> GSMDEQEALNSIMNDLVALQMNRRHRMPGY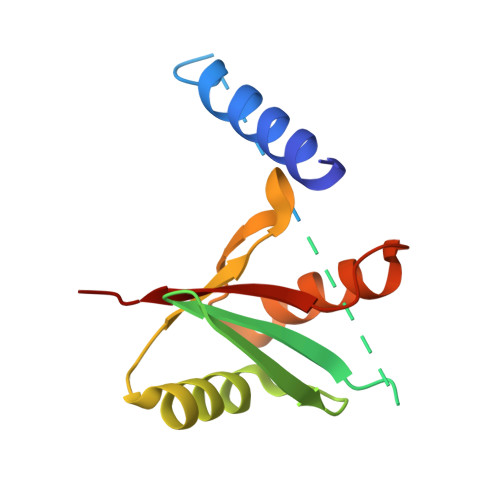ETMKNKDTGHSNRQSDVRIKFEHNGERRIIAFSRPVKYEDVEHKVTTVFGQPLDLHYMNNELSILLKNQDDLDKAIDILDRSSSMKSLRILLLSQD> GPGTTDQPLAKDKVALLIGNMNYREHPKLKAPLVDVYELTNLLRQLDFKVVSLLDLTEYEMRNAV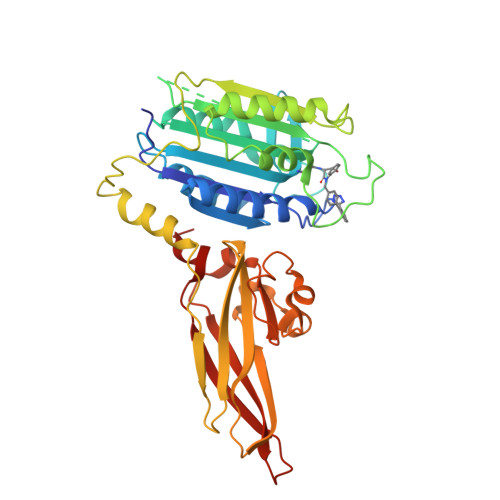DEFLLLLDKGVYGLLYYAGHGYENFGNSFMVPVDAPNPYRSENCLCVQNILKLMQEKETGLNVFLLDMCRKRNDYDDTIPILDALKVTANIVFGYATCQGAEAFEIQHSGLANGIFMKFLKDRLLEDKKITVLLDEVAEDMGKCHLTKGKQALEIRSSLSEKRALTDPIQGTEYSAESLVRNLQWAKAHELPESMCLKFDCGVQIQLGFAAEFSNVMIIYTSIVYKPPEIIMCDAYVTDFPLDLDIDPKDANKGTPEETGSYLVSKDLPKHCLYTRLSSLQKLKEHLVFTVCLSYQYSGLEDTVEDKQEVNVGKPLIAKLDMHR> MLKLAIPKGRLEEKVMTYLKKTGVIFERESSILREGKDIVCFMVRPFDVPTYLVHGVADIG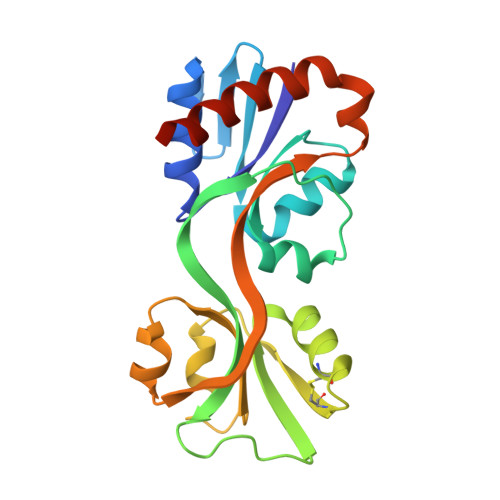FCGTDVLLEKETSLIQPFFIPTNISRMVLAGPKGRGIPEGEKRIATKFPNVTQRYCESKGWHCRIIPLKGSVELAPIAGLSDLIVDITETGRTLKENNLEILDEIFVIRTHVVVNPVSYRTKREEVVSFLEKLQEVIEHDSNEQSRG2,2-dimethyl-4-oxidanylidene-pentanedioic acid | C7 H10 O5 | 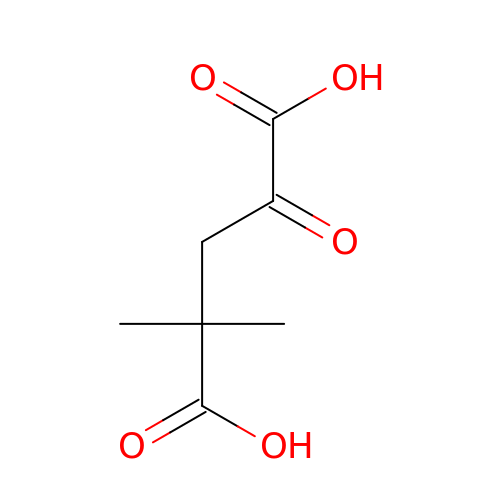UMLBANZGNKNTIS-UHFFFAOYSA-N methyl 3-O-[(1R)-1-carboxyethyl]-beta-D-galactopyranoside 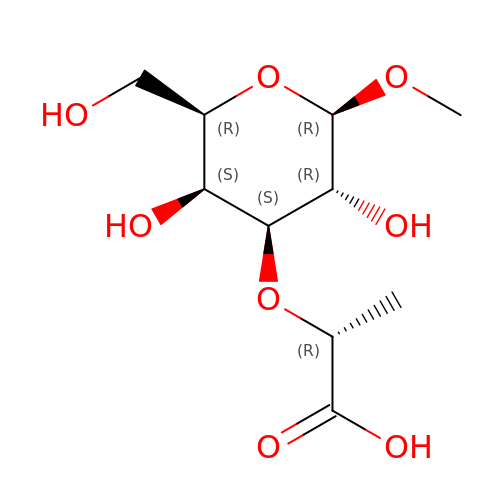| C10 H18 O8 | PXMURYZLIUEKLA-BEESJRNYSA-N> MRWSAVLCKVSKVPTRSVIPADALRYHPRYSVPRKMVLSNTFNVVGENNRYTSLKLILEK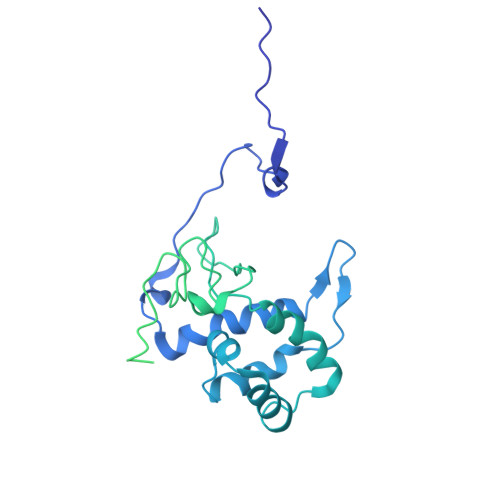LSGHVGRRQYKMLCNLEKHYDKLKDEGIDWHELKWLSREELIVLFDKVLHLTRTERAALLPAIEAKVCGVLRQTDSRHSTVVCMNRGNANHGWRCGRNGHTNDVYFEGKAKANTAALQLCRRSSVRSVERSGVLVEVRSEPDFSVVGRFDHSLSPRVWSTPENPTFQVTTIGYEFRVHQEDPRVIPQIVEAAEEWELHANITKQVIWEMLEMYAVERDRQPLDLKPGEMGDPDIPSRHATAFNVQVVPPLSEGDEAIQVVEQRIVRADGSEVPWFQEPPPQLFSGGIPVILPFAPSIIVKSTFRQVTRSSAQDVTRQLLQPVVDVTCFLHPNVCFWWNAEDEQRCLGHIVDYAKRIPFALPFNLYFRVNLSKDLRGVQNYTEELGKRMSMKAHYFNLRSYGVR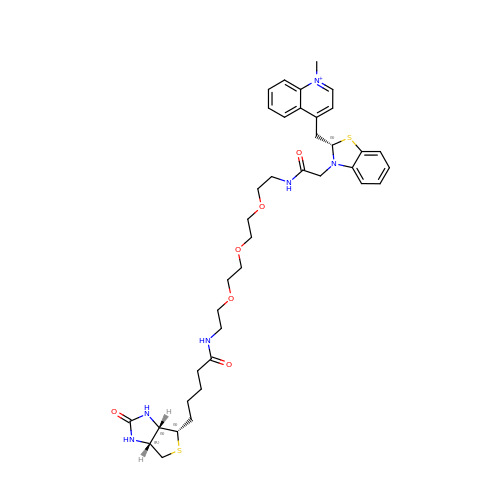4-{[(2S)-3-{2,16-dioxo-20-[(3aS,4S,6aR)-2-oxohexahydro-1H-thieno[3,4-d]imidazol-4-yl]-6,9,12-trioxa-3,15-diazaicosan-1-yl}-2,3-dihydro-1,3-benzothiazol-2-yl]methyl}-1-methylquinolin-1-ium | C38 H51 N6 O6 S2 | BXBHTLUUPXOIJA-SDUHKGLLSA-O>MGACPPKAKGPWAQLQKLLISWPVGEQDWEQYRDRVNMLQQERIRDSPLLQAAKENDLRLLKILLLNQSCDFQQRGAVGETALHVAALYDNLEAATLLMEAAPELAKEPALCEPFVGQTALHIAVMNQNLNLVRALLARGASVSARATGAAFRRSPHNLIYYGEHPLSFAACVGSEEIVRLLIEHGADIRAQDSLGNTVLHILILQPNKTFACQMYNLLLSYDEHSDHLQSLELVPNHQGLTPFKLAGVEGNTVMFQHLMQKRKHVQWTCGPLTSTLYDLTEIDSWGEELSFLELVVSSKKREARQILEQTPVKELVSFKWKKYGRPYFCVLASLYILYMICFTTCCIYRPLKLRDDNRTDPRDITILQQKLLQEAYVTHQDNIRLVGELVTVTGAVIILLLEIPDIFRVGASRYFGQTILGGPFHVIIITYASLVLLTMVMRLTNMNGEVVPLSFALVLGWCSVMYFARGFQMLGPFTIMIQKMIFGDLMRFCWLMAVVILGFASAFHITFQTEDPNNLGEFSDYPTALFSTFELFLTIIDGPANYSVDLPFMYCITYAAFAI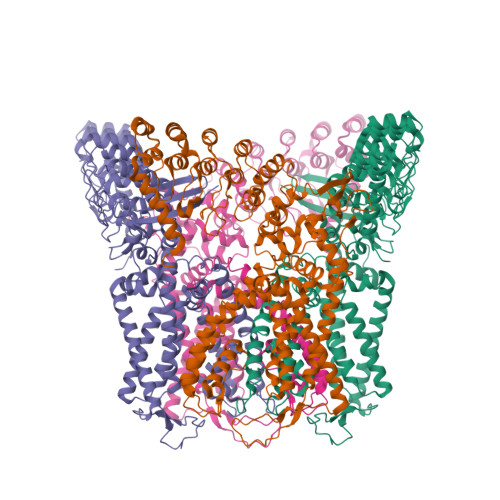IATLLMLNLFIAMMGDTHARVAQERDELWRAQVVATTVMLERKMPRFLWPRSGICGYEYGLGDRWFLRVENHHDQNPLRVLRYVEAFKCSDKEDGQEQLSEKRPSTVESGMLSRASVAFQTPSLSRTTSQSSNSHRGWEILRRNTLGHLNLGLDLGEGDGEEVYHF[4x]>[2x]MKPARPCL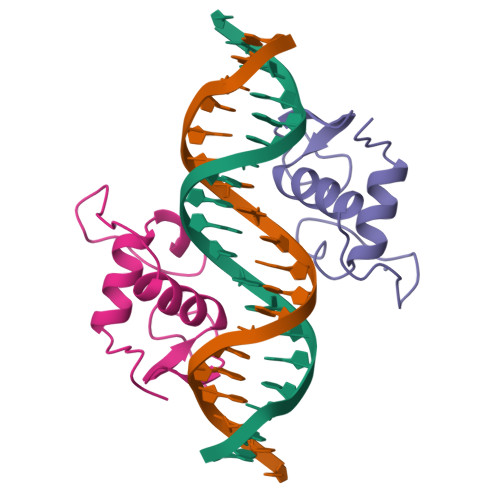VCSDEASGCHYGVLTCEGCKAFFKRAVEGQHNYLCKYEGKCIIDKIRRKNCPACRYRKCLQAGMNLEARKTKKK~{N}-[[(3~{R})-1-[6-(3~{H}-benzimidazol-4-ylmethylamino)pyrimidin-4-yl]-3-oxidanyl-piperidin-3-yl]methyl]-4-[(4,4-dimethylpiperidin-1-yl)methyl]benzamide | C33 H42 N8 O2 | 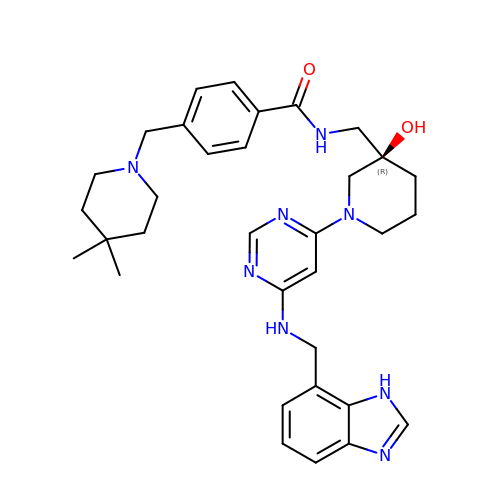IASLOXMPEUOUSU-MGBGTMOVSA-N> MELK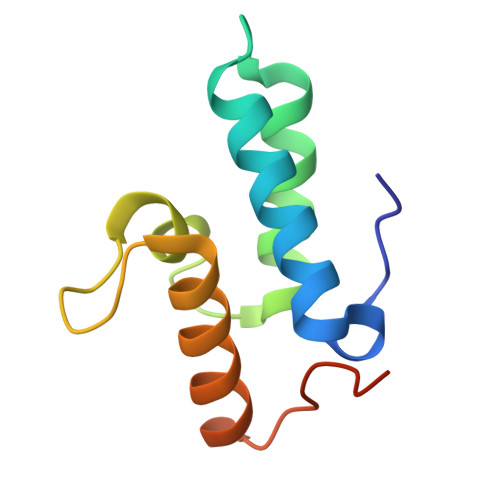NSISDYTEAEFVQLLKEIEKENVAATDDVLDVLLEHFVKITEHPDGTDLIYYPSDNRDDSPEGIVKEIKEWRAANGKPGFKQGHHHHHH4-(2-phenoxyethanoyl)piperazin-2-one 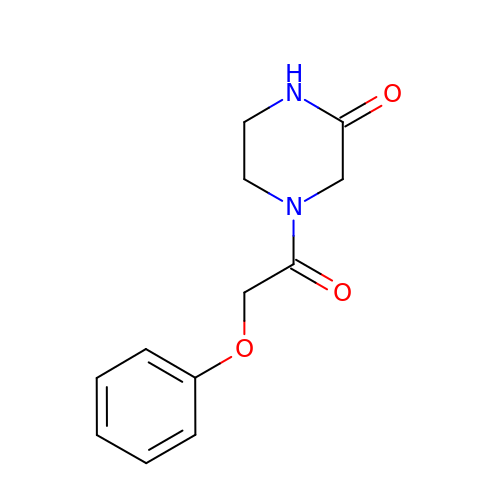| C12 H14 N2 O3 | VQOCCTAPSDVOOO-UHFFFAOYSA-N> TDPDPLQDFCVADLDGKAVSVNGHTCKPMSEAG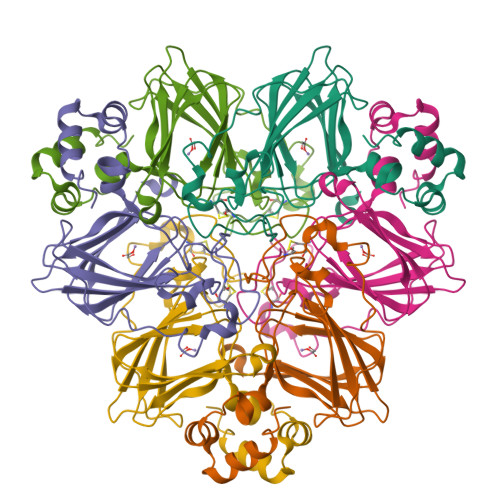DDFLFSSKLTKAGNTSTPNGSAVTELDVAEWPGTNTLGVSMNRVDFAPGGTNPPHIHPRATEIGMVMKGELLVGILGSLDSGNKLYSRVVRAGETFVIPRGLMHFQFNVGKTEAYMVVSFNSQNPGIVFVPLTLFGSDPPIPTPVLTKALRVEAGVVELLKSKFAGGS Cohesion is facilitated by cohesin, a member of the Structural Maintenance of Chromosomes (SMC) family of protein complexes, which is responsible for genome organisation across all domains of life. Cohesin complexes form tripartite rings, comprising Smc1-Smc3 and the kleisin subunit Scc1, that are proposed to topologically entrap sister DNA molecules. We show here that cohesin interacts directly with DNA through a complex formed by the HEAT-repeat subunit Scc3 and the kleisin subunit Scc1. In addition to providing a scaffold for the assembly of cohesin regulators and thereby participating in the maintenance of cohesion, the Scc3-Scc1 subcomplex also plays a key role in DNA substrate recognition and hence the efficient association of the cohesin holocomplex with chromatin.

To identify the molecular basis of this interaction, we crystallized the Scc3T-Scc1K complex from budding yeast bound to 19 bp of dsDNA. Optimized crystals diffracted anisotropically to a minimum Bragg spacing of 3.6 Å in the best, and ~5.7 Å in the worst direction. Despite these drawbacks, we successfully traced the structure using a selenomethionine derivative and refined a model encompassing amino acid residues 134 to 1064 of Scc3 in complex with residues 309 to 400 of Scc1, bound to a 19 bp DNA molecule. As seen in other structures of Scc3, the protein is hook-shaped in the C-terminal section and contains an N-terminal ‘nose’ formed by a pair of extended antiparallel α-helices. Similarly to the interaction of human Scc1 with Scc3, the yeast Scc1 in our structure binds along the convex surface of the hook-shaped HEAT-repeat subunit. We detected additional electron density corresponding to dsDNA within the cradle of this hook. To identify amino acid residues potentially involved in DNA binding, we mapped the electrostatic surface potential onto the Scc3-Scc1 structure. This revealed that DNA is nested within an extended cradle spanning the majority of Scc3-Scc1, lined by a set of positively charged residues that directly contact the DNA phosphate backbone. We observed no direct nucleotide base–amino acid interactions, which explains the apparent lack of DNA sequence specificity. We conclude that the positively charged Scc3 cradle comprises the major DNA-binding surface of Scc3 and that the positively charged amino acid residues located in patch 1 and 3 constitute a composite DNA binding surface. We conclude that DNA binding by Scc3-Scc1 is essential for the stable association of cohesin complexes with chromosomes in vivo and hence an important determinant of cohesin function.

>[2x]MTAVRRSTRIRTKSQVIEEDYDDEQNTSAQHVESDKITAKTQHEEEEEQDTGESEESSSEDDYEDQDDDDYVDTATAKRKSRKRKPKSASNTSSKRQKKKPTSAQKSAVSHAPAYHRSKKDQDQYLEIAKDFQPTELFDILSTSEDVSIEELLREWLETYSENRDKFLQEFINLLLNCCGSVARVEDHDVHSNESSNETIGEIQLLFQRQKLHEFYLLISKENKKRKNFKMGPLYQNFAEFMTKLLEVANDLQLLYVESDEDDTQIVTGNLVLDLLTWLSSFSVCKIRCFRYISTLTLYLFQDYLTQQAVNLEKNYLAKLSKQLSLEEKKKRPNNKTLEKLESTIAETQGSKVVIDSIIDNIVKLCFVHRYKDVSDLIRSESMLHLSIWIKNYPEYFLKVTFLKYFGWLLSDNSVSVRLQVTKILPHLIIQNHNSKSTDNSAIRQVFERFKTKILEVAIRDVNLDVRIHSIQVLTEASSLGYLDDSEILIISSLMFDEEFDPFKTSSFNKRSKFLSTVAKFLARVIKEKFDEFIKTHEDLPKEVDGLEVGPVVQVGIFIKILNDSLIYHLKDCAEVDSRTKIRMLTQAAEFLSPYISTHLKTICNLLISDTESNELIQKLQNSANNNSDDEDVDDEELDITPLFPIDRNSTILYLNVFHGLCAGANNPKIQTKDSVKEIVLPLFYDLLNAASIESADILCPLLESFITFSLDDWISIGYETELKKITDKTIKAFMDSTIGNSKVDMKYDIFAKFIHHIHHFEKKELQEKFLNQIATLKIHLKKFLQEKMDPNNSRDDYKDLTCSLYELYINKLTILGRDYPIEVDEELLQLFLNNFVSRIPIMFQDFDDSTAQEINFKMLVLLATWNLEKWREIIEKVRDYENSISKDLRSVWKPIAAIIGRLNTLVISLAATNETFENINSLFYLKWSACTSLMDIIVAIKIFELKLPADATTWRYSMSEQFPFYLHDNASKVLLKIFLYLESLFAKQVDVQLERVADEDANLNDLPETGFFENIETEFLLFTVKLKGLMKLNILDERFASRVALNKEKLGPLFKKIVDDTIMENPEPNKKNIQKAKSNQTQREKAPLQPNSERETDHANTENNDPDIPMTIDLEPIEESSQNNSELAPIEEHPTVVDAIDNSDEITQD;>TDAMTESQPKQTGTRRNSKLLNTKSIQIDEETENSESIASSNTYKEERSNNLLTPQPTNFTTKRLWSEITESMSYLPDPILKNFLSYESLKKRKIHNGRE[2x]>MRVLLIAGGVSPEHEVSLLSAEGVLRHIPFPTDLAVIAQDGRWLLGEKALTALEAKAAPEGEHPFPPPLSWERYDVVFPLLHGRFGEDGTVQGFLELLGKPYVGAGVAASALCMDKDLSKRVLAQAGVPVVPWVAVRKGEPPVVPFDPPFFVKPANTGSSVGISRVERFQDLEAALALAFRYDEKAVVEKALSPVRELEVGVLGNVFGEASPVGEVRYEAPFYDYETKYTPGRAELLIPAPLDPGTQETVQELALKAYKVLGVRGMARVDFFL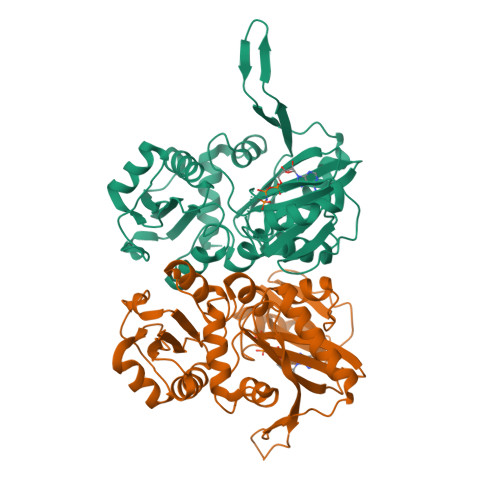AEGELYLNELNTIPGFTPTSMYPRLFEAGGVAYPELLRRLVELALT[3x]>[2x]ALVXFAE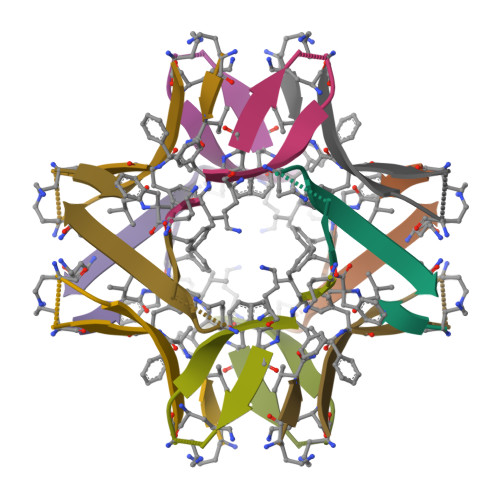DAAIIGLAV> AGTAWAQDADKLPHTKVTLVAPPQVHPHEQATKSGPKVVEFTMTIEEKKMVIDDKGTTLQAMTFNGSMPGPTLVVHEGDYVQLTLVNPATNAMPHNVDFHGATGALGGAKLTNVNPGEQATLRFKADRSGTFVYHCAPEGMVPWHVVSGMSGTLMVLPRDGLKDPQGKPLHYDRAYTIGEFDLYIPKGPDGKYKDYATLAESYGDTVQVMRTLTPSHIVFNGKVGALTGADALTAKVGETVLLIHSQANRDTRPHLIGGHGDWVWETGK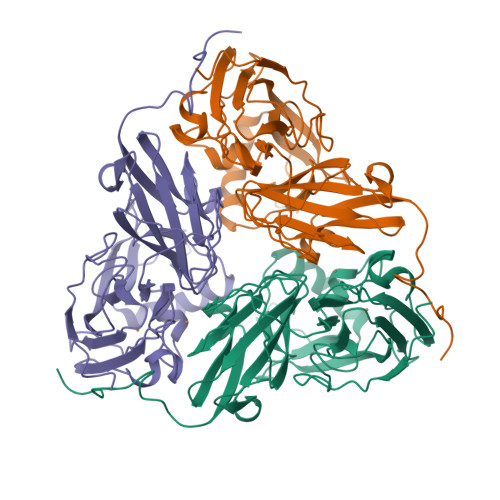FANPPQRDLETWFIRGGSAGAALYTFKQPGVYAYLNHNLIEAFELGAAGHIKVEGKWNDDLMKQIKAPAPIPR>[2x]SNAMFADTAALKAAMDTAL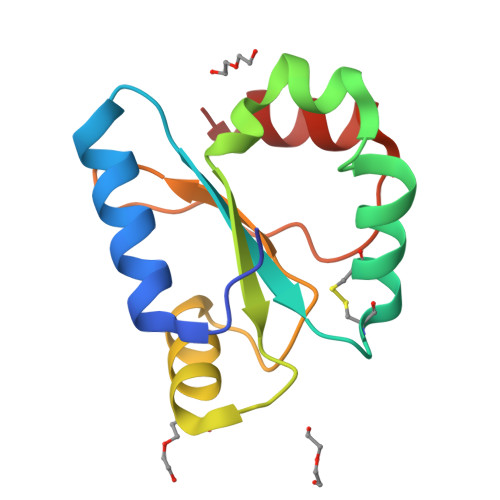KEHPDKPVVLDFYADWCISCKEMAAYTLNQPEVHQAVDMERFFQIDVTANTPEHQALLKEYGLFGPPGVFVVRSDGSRSEPLLGFVKADKFIEWYEQNR> MGHHHHHARSVRHIAIPAHRGLITDRNGEPLAVSTPVTTLWANPKELMTAKERWPQLAAALGQDTKLFADRIEQNAEREFIYLVRGLTPEQGEGVIALKVPGVYSIEEFRRFYPAGEVVAHAVGFTDVDDRGREGIELAFDEWLAGVPGKRQVLKDRRGRVIKDVQVTKNAKPGKTLALSIDLRLQYLAHRELRNALLENGAKAGSLVIMDVKTGEILAMTNQPTYNPNNRRNLQPAAMRNRAMIDVFEPGSTVKPFSMSAALASGRWKPSDIVDVYPGTLQIGRYTIRDVSRNSRQLDLTGILIKSSNVGISKIAFDIGAESIYSVMQQVGLGQDTGLGFPGERVGNLPNHRKWPKAETATLAYGYGLSVTAIQLAHAYAALANDGKSVPLSMTRVDRVPDGVQVISPEVASTVQGMLQQVVEAQGGVFRAQVPGYHAAGKSGTARKVSVGTKGYRENAYRSLFAGFAP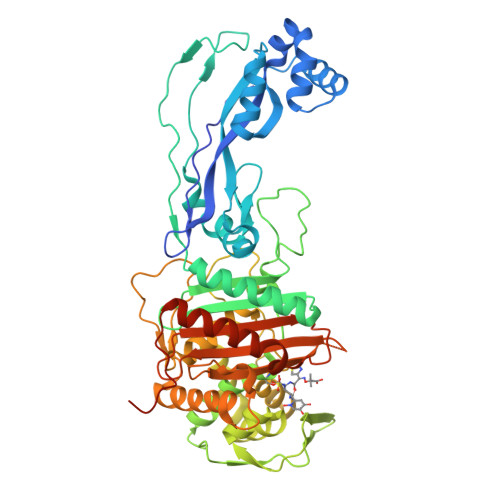ATDPRIAMVVVIDEPSKAGYFGGLVSAPVFSKVMAGALRLMNVPPDNLPTATEQQQVNAAPAKGGRG>[2x]MLVWLAEHLVKYYSGFNVFSYLTFRAIVSLLTALFISLWMGPRMIAHLQKLSFGQVVRNDGPESHFSKRGTPTMGGIMILTAIVISVLLWAYPSNPYVWCVLVVLVGYGVIGFVDDYRKVVRK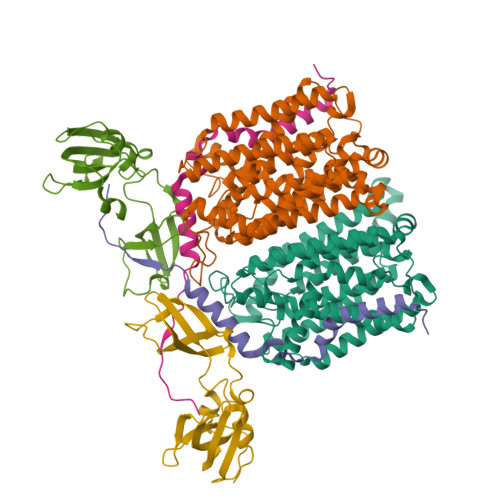DTKGLIARWKYFWMSVIALGVAFALYLAGKDTPATQLVVPFFKDVMPQLGLFYILLAYFVIVGTGNAVNLTDGLDGLAIMPTVFVAGGFALVAWATGNMNFASYLHIPYLRHAGELVIVCTAIVGAGLGFLWFNTYPAQVFMGDVGSLALGGALGIIAVLLRQEFLLVIMGGVFVVETLSVILQVGSFKLRGQRIFRMAPIHHHYELKGWPEPRVIVRFWIISLMLVLIGLATLKVR;>[2x]MGHWTLSGILAFLLLLSLLLPSLLIMFIPLTFRRPASSWKARSLQKILLMASSVRLKPLSSSRIPCVLRPDSKRRFHHHHHH;>[2x]MKVAKDLVVSLAYQVRTEDGVLVDESPVSAPLDYLHGHGSLISGLETALEGHEVGDKFDVAVGANDAYGQYDENLVQRVPKDVFMGVDELQVGMRFLAETDQGPVPVEITAVEDDHVVVDGNHMLAGQNLKFNVEVVAIREATEEELAHGHVHG>MKRPKVSIVGAGNTGAALAHWLAIKQVADIVLVDVVEGMPQGKALDLMQSAPVEGFDVVITGSNDYAATAGSDVVVITAGAARKPGMSRDDLVNINTGIVREITAQVARYSPDAYLIVLTNPLDVMCYVAYKVSGFPKHRVMGQSGILDSARFRTFIARELNVSFED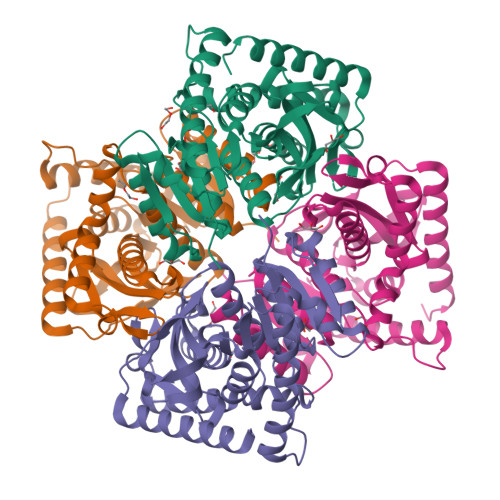VHALVLGGHGDSMVPLPRYTHVGGIPVTQLLPKEKIDELVRRTRDGGAEIVRLLKTGSAFFAPGAAMAEMVEAILRDRKRVLPVSAYLEGEYGESGIFMGVPVVLGGNGIEKILEIELTDEERQAFARSAADVRQTLSKLDL[4x]>MFEQRVNSDVLTVSTVNSQDQVTQKPL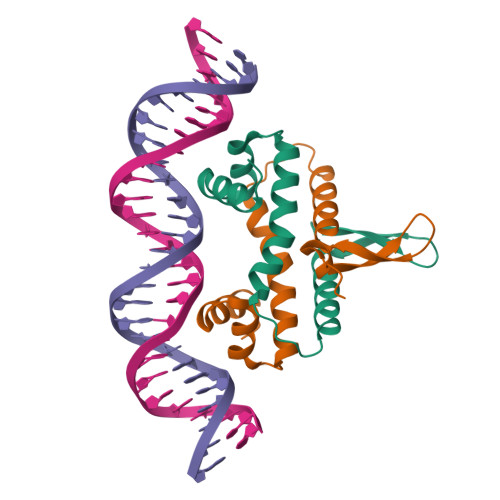RDSVKQALKNYFAQLNGQDVNDLYELVLAEVEQPLLDMVMQYTRGNQTRAALMMGINRGTLRKKLKKYGMN[2x]(2E)-4-fluoro-3-methylbut-2-en-1-yl trihydrogen diphosphate | C5 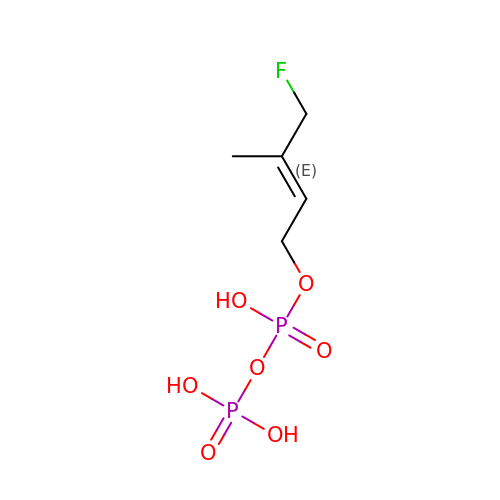H11 F O7 P2 | OAODEACEICJXDG-GORDUTHDSA-N>GPLGSYSHTATPAITLPSSGSANFAGVEYPLLPLDQHTPLLFQWFERNPSRFGENQIPIINTQQNPYLNNIINAAIIEKERTIGVLVDGNFSAGQKKALAKLEKQYENIKVI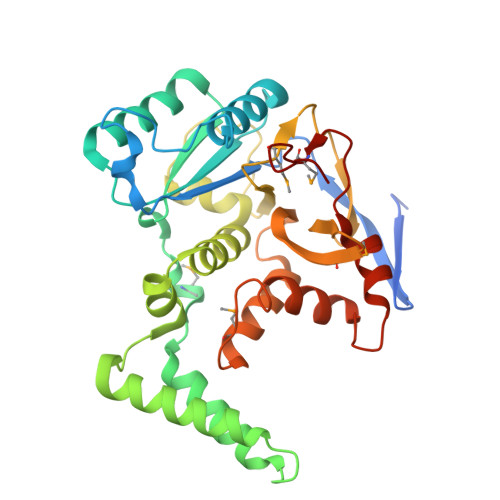YNSDLDYSMYDKKLSDIYLENIAKIEAQPANVRDEYLLGEIKKSLNEVLKNNPEESLVSSHDKRLGHVRFDFYRNLFLLKGSNAFLEAGKHGCHHLQPGGGCIYLDADMLLTGKLGTLYLPDGIAVHVSRKGNSMSLENGIIAVNRSEHPALKKGLEIMHSKPYGDPYIDGVCGGLRHYFNCSIRHNYEEFCNFIEFKHEHIFMDTSSLTISS[2x]>[2x]SNAMSQFMNLEGKVALVTGASRGIGKAIAELLAERGAKVIGTATSESGAQAISDYLGDNGKGMALNVTNPESIEAVLKAITDEFGGVDILVNNAGITRDNLLMRMKEEEWSDIMETNLTSIFRLSKAVLRGMMKKRQGRIINVGSVVGTMGNAGQANYAAAKAGVIGFTKSMAREVASRGVTVNT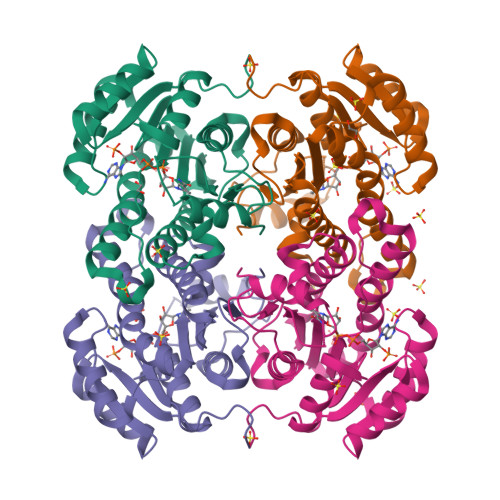VAPGFIETDMTKALNDEQRTATLAQVPAGRLGDPREIASAVAFLASPEAAYITGETLHVNGGMYMI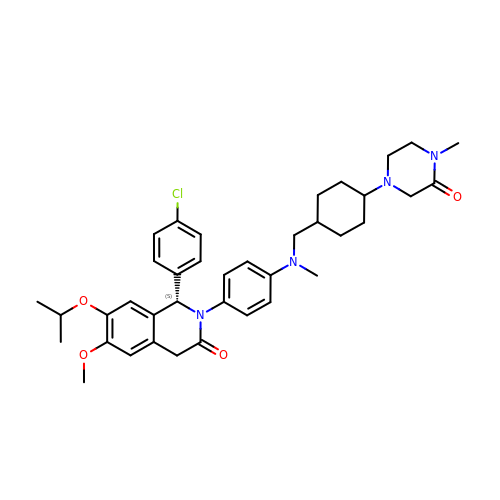(S)-1-(4-chlorophenyl)-7-isopropoxy-6-methoxy-2-(4-(methyl(((1r,4S)-4-(4-methyl-3-oxopiperazin-1-yl)cyclohexyl)methyl)amino)phenyl)-1,2-dihydroisoquinolin-3(4H)-one | C38 H47 Cl N4 O4 | CLRSLRWKONPSRQ-IIPSPAQQSA-N> MSRAYDLVVLGAGSGGLEAGWNAAVTHKKKVAVVDVQATHGPPLFAALGGTCVNVGCVPKKLMVTGAQYMDLIRESGGFGWEMDRESLCPNWKTLIAAKNKVVNSINESYKSMFADTEGLSFHMGFGALQDAHTVVVRKSEDPHSDVLETLDTEYILIATGSWPTRLGVPGDEFCITSNEAFYLEDAPKRMLCVGGGYIAVEFAGIFNGYKPCGGYVDLCYRGDLILRGFDTEVRKSLTKQLGANGIRVRTNLNPTKITKNEDGSNHVHFNDGTEEDYDQVMLAIGRVPRSQALQLDKAGVRTGKNGAVQVDAYSKTSVDNIYAIGDVTNRVMLTPVAINEGAAFVETVFGGKPRATDHTKVACAVFSIPPIGTCGMTEEEAAKNYETVAVYASSFTPLMH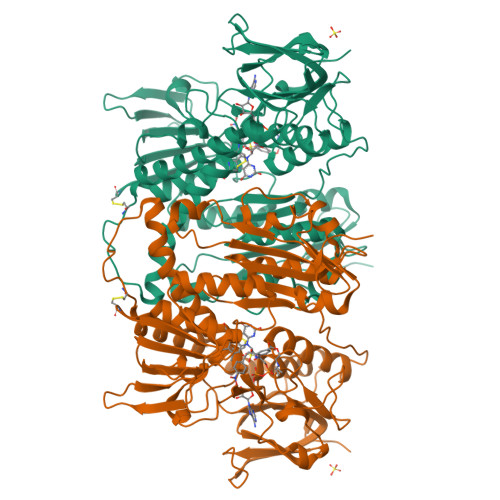NISGSKHKEFMIRIITNESNGEVLGVHMLGDSAPEIIQSVGICMKMGAKISDFHSTIGVHPTSAEELCSMRTPAYFYESGKRVEKLS> WQPPWYAKEP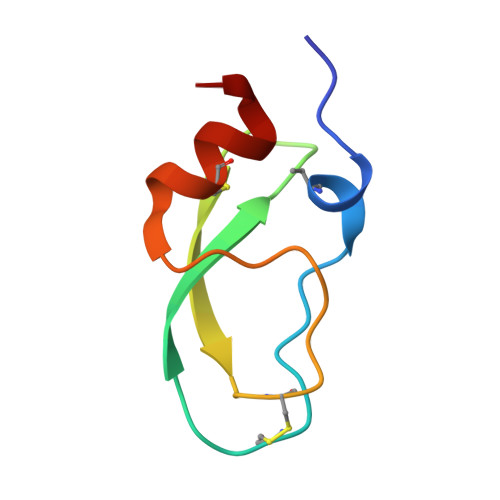VRIGSCKKQFSSFYFKWTAKKCLPFLFSGCGGNANRFQTIGECRKKCLGK The inwardly rectifying potassium channels (Kir channels) regulate membrane electrical excitability and K+ transport in a wide range of cell types. Kir channel activity is controlled by dynamic conformational changes that regulate the flow of K+ ions through the central pore of the channel. KirBac3.1, Kir6.2, and Kir6.1 channels are homotetramers of four subunits. Each subunit has a transmembrane domain (TMD), containing an outer transmembrane helix (TM1), a selectivity filter (SF), and an inner transmembrane helix (TM2).

The tryptophan at position 46 in KirBac3.1, corresponding to W68 in Kir6.2, located at the cytosolic end of transmembrane helix 1 (TM1), is highly conserved within the inward rectifying potassium channel family, suggesting that it has a critical role. In this paper, we present the crystal structure of the KirBac3.1 W46R mutant channel (homologous to the human Kir6.2 channel) at 2.80 Å and provide a structural and functional characterization using a multi-technique approach. We grew crystals of the W46R mutant belonging to space group P21212. The structure was solved by molecular replacement, and a final model containing 279 out of the 301 residues of the construct was refined to an R-factor of 22.2% and an R-free of 28.7%, with 99.3% of the residues in the final model lying either in the most favorable or in the allowed regions of the Ramachandran plot. The mutation replaces a tryptophan residue that is highly conserved across the Kir family to an arginine, disrupts the contacts between the outer (TM1) and inner (TM2) helices, and creates new contacts shown in our crystallographic data. The atomic structure of the W46R mutant shows that the four R46 side chains point away from the channel pore and are engaged in intersubunit connections with residues Y38 and D36 on the slide helix of the adjacent subunit (n − 1: counterclockwise neighbor chain). The interactions between the flipped-in W46 residue and the two R134 and F135 residues at the bottom of the TM2 are lost in the case of the W46R due to the orientation of the mutated residue R46 toward the outside of the channel. The HDX studies show that the only region that is less flexible compared with the WT structure is at the cytoplasmic bottom end of the TM1, including the R46 mutation, suggesting that the network of interactions formed between the mutated residue R46 and the slide helix increases the rigidity of this protein segment.

>[2x]MTGGMKPPARKPRILNSDGSSNITRLGLEKRGWLDDHYHDLLTVSRPVFITLITGLYLVTNALFALAYLACGDVIENARPGSFTDAFFFSVQTMATIGYGKLIPIGPLANTLVTLEALCGMLGLAVAASLIYARFTRPTAGVLFSSRMVISDFEGKPTLMMRLANLRIEQIIEADVHLVLVRSEISQEGMVFRRFHDLTLTRSRSPIFSLSWTVMHPIDHHSPIYGETDETLRNSHSEFLVLFTGHHEAFAQNVHARHAYSCDEIIWGGHFVDVFTTLPDGRRALDLGKFHEIAQHHHHHH> MAEQATKSVLFVCRGNKCRSPIAEAVFRKLVTDQNISENWVIDSGAVSDWNVGRSPDPRAVSCLRNHGIHTAHKARQITKE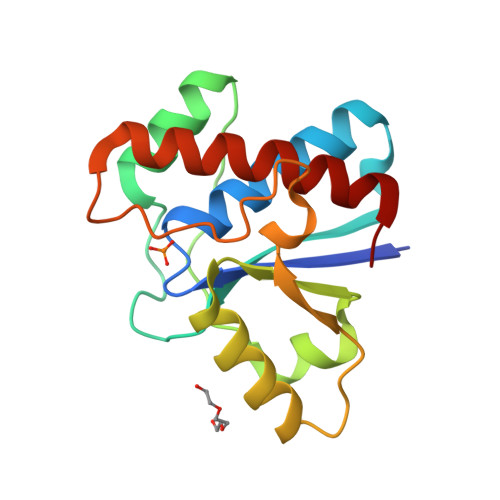DFATFDYILCMDESNLRDLNRKSNQVKTCKAKIELLGSYDPQKQLIIEDPYYGNDSDFETVYQQCVRCCRAFLEKAH> RLHFMQVDSVQRWMED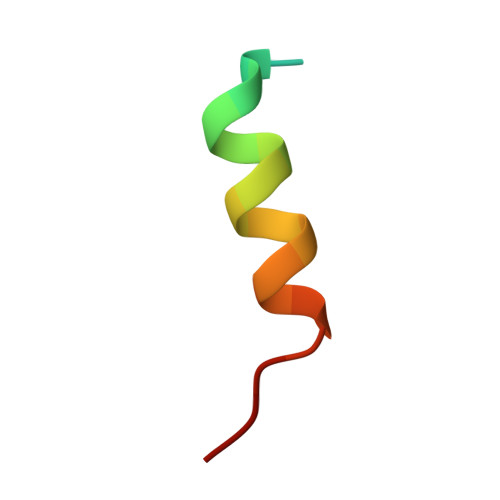LKLMTE>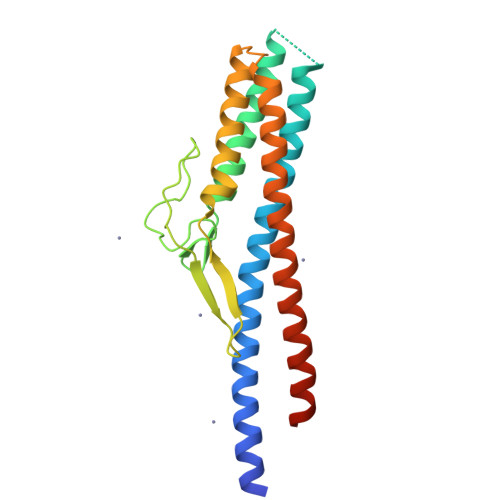[2x]GSAKDPAASKSFAIQHSLANMEQMQKDIADSKNVLTQTENTLQGVLKSLTRADQLTVQALNGTNSEKELQAIGVEIDQILKQVVYLANTKEQGRYIFGGDSAENLPFTEDGTYQGGKNDVNWKLNDGYEFKAFRNGEALLSPVIKTLKQMSEAMQNGDQKALKPLLEENKQNLDGIINRTTEVGSTMNTMETFKTILSEQNVALQENRKEIED The human proteome comprises 266 human PDZ (PSD95/DLG1/ZO1) domains 16 and about 4000 putative PBMs, defining a network of one million potential interactions. PBMs are mostly (though not exclusively) C-terminal, with their COO- implicated in binding, and are classified based on position −2, being respectively Ser/Thr, hydrophobic or acidic in classes 1, 2, and 3 17,18. PDZ-PBM interactions are rather transient and promiscuous. Viral proteins bearing functional PBMs are found notably in HPV and HTLV oncoviruses as well as in HBV, WNV and coronaviruses including MERS or SARS-CoV213,15,23–26.

In another example, the profile and the logo of SYNJ2BP indicate that this PDZ-domain is highly promiscuous, with however a mild preference for E-T-x-V-COO- motifs and a moderate bias for basic residues at upstream (−4 and −5) positions. F HTLV Tax1 PBM sequence matches strongly with SYNJ2BP logo at p0, p-1, p-2, p-3, and p-4. Accordingly, Tax1 is the strongest SYNJ2BP binder in our interactome. In the structure of HTLV1 Tax1 PBM bound to SYNJ2BP, p-3 Glu of Tax1 engages contacts reminiscent of those of p-3 phospho-Ser of RPS6KA1, confirming SYNJ2BP’s preference for a negative p-3. In the SYNJ2BP-Tax1 complex, Glu at p-3 of Tax1 engages similar contacts as pSer of RPS6KA1_−3P, while Arg at p-4 provides additional contact to the α2 helix of SYNJ2BP. Yet Tax1 matches better than phosphorylated RPS6KA1 to SYNJ2BP’s logo thanks to a basic p-4 Arg and a p0 Val (Pro and Leu in RPS6KA1, respectively). Accordingly, in the crystal structures, p-4 Arg of Tax1 establishes favorable H-bonds with a Gln from the α2 helix of SYNJ2BP PDZ, and the Val-bound state of SYNJ2BP PDZ is more compact than its Leu-bound state, due to displacement of the carboxylate-binding GLGF loop likely driven by the larger side-chain of Leu. G Superposition of Tax1 and p-3 phosphorylated RPS6KA1 PBMs bound to SYNJ2BP.

> GSHMDYLVTEEEINLTRGPSGLGFNIVGGTDQQYVSNDSGIYVSRIKENGAAALDGRLQEGDKILSVNGQDLKNLLHQDAVDLFRNAGYAVSLRVQHRLQVQGSAYGSVKAYTNFDAERDALNIETAIKTKGVDEVTIVNILTNRSNEQRQDIAFAYQRRTKKELASALKSALSGHLETVILGLLKTPAQYDASELKASMKGLGTDEDSLIEIICSRTNQELQEINRVYKEMYKTDLEKDIISDTSGDFRKLMVALAKGRRAEDGSVIDYELIDQDARDLYDAGVKRKGTDVPKWISIMTERSVPHLQKVFDRYKSYSPYDMLESIRKEVKGDLENAFLNLVQCIQNKPLYFADRLYDSMKGKGTRDKVLIRIMVSRSEVDMLKIRSEFKRKYGKSLYYYIQQDTKGDYQKALLYLCGGDD;> TDDSEKHFRETEV> MDNREIVMKYISYKLSQRGYEWDAG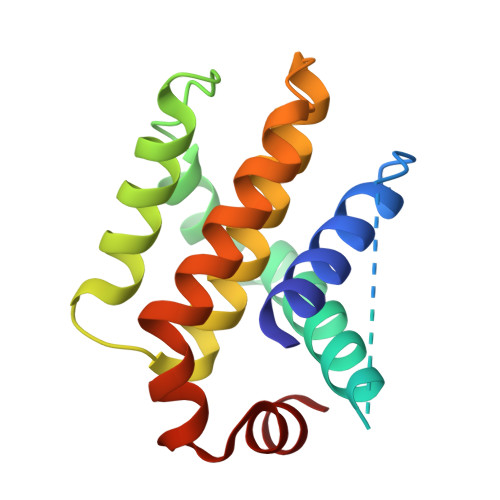DVEENRTEAPEGTESEVVHQTLRQAGDDFSLRYRRDFAEMSSQLHLTPGTAYASFATVVEELFRDGVNWGRIVAFFEFGGVMCVESVNREMSVLVDNIAAWMATYLNDHLHTWIQDNGGWDAFVELYG> MELCTHLSYSRSLSPGKAVFFYKTAESDFVPLRI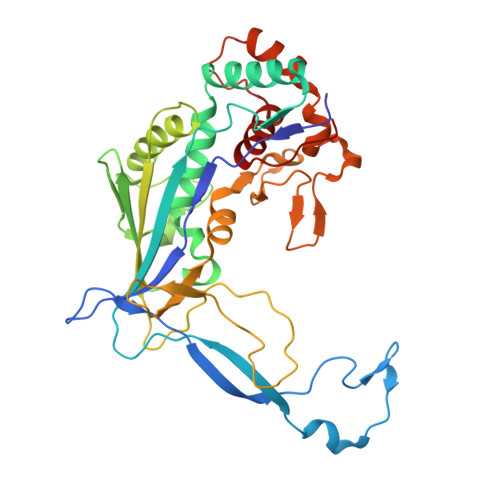EVAKISGQKCGYTEGFDANLKPKNIERYELAYSNPQTIEACYVPPNVDELYCRFSLRVEANSMRPYVCSNPDVLRVMIGLAQAYQRLGGYNELARRYSANVLRGIWLWRNQYTQGTKIEIKTSLGSTYHIPDARRLSWSGDWPELEQKQLEQLTSEMAKALSQPDIFWFADVTASLKTGFCQEIFPSQKFTERPDDHSVASRQLATVECSDGQLAACINPQKIGAALQKIDDWWANDADLPLRVHEYGANHEALTALRHPATGQDFYHLLTKAEQFVTVLESSEGGGVELPGEVHYLMAVLVKGGLFQKGKGR>MDGSGEQPRGGGPTSSEQIMKTGALLLQGFIQDRAGRMGGEAPELALDPVPQDASTKKLSESLKRIGDELDSNMELQRMIAAVDTDSPREVFFRVAADMFSDGNFNWGRVVALFYFASKLVLKALSTK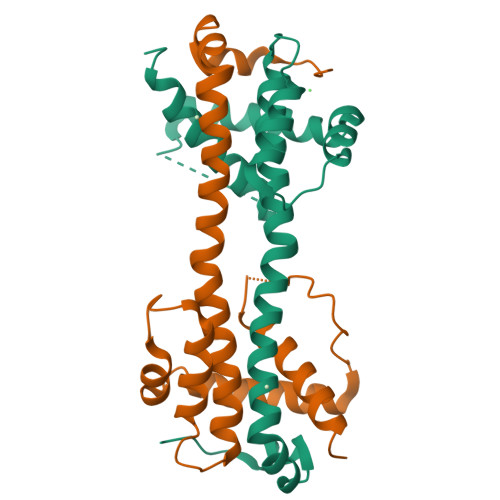VPELIRTIMGWTLDFLRERLLGWIQDQGGWDGLLSYFGTPTWQGSS[4x]SPERMINE (FULLY PROTONATED 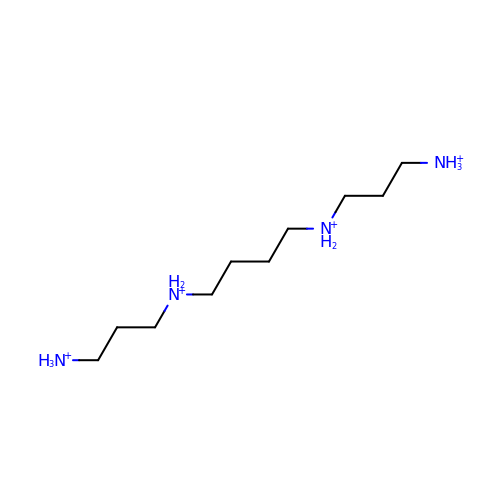FORM) | C10 H30 N4 | PFNFFQXMRSDOHW-UHFFFAOYSA-R> MSYCTLADLIEQYSEQKIREVSDRVNKPATTIDTVIVDRAIADADSEIDLHLHGR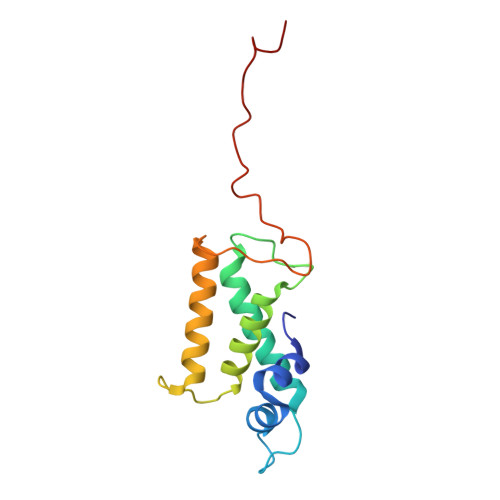YQLPLASVPTALKRIACGLAYANLHIVLKEENPVYKTAEHLRKLLSGIANGKLSLALDADGKPAPVANTVQISEGRNDWGADW SNARE (soluble N-ethylmaleimide-sensitive factor (NSF) attachment protein receptor) proteins drive membrane fusion at different cell compartments as their core domains zipper into a parallel four-helix bundle. After fusion, these bundles are disassembled by the AAA+ (ATPase associated with diverse cellular activities) protein Sec18/NSF and its adaptor Sec17/α-SNAP to make them available for subsequent rounds of membrane fusion. The disassembly requires multiple ATP hydrolysis events in the presence of Mg2+; as few as six ATP hydrolysis events are sufficient. The side-loading and side-release mechanism explains how Sec18/NSF can disassemble SNAREs with constrained topologies.

Next, we asked whether this same side opening of Sec18 occurs in the hydrolyzing condition without SNARE substrate. We prepared purified wild-type Sec18 in the presence of ATP and Mg2+ in a three-stage procedure that yielded a pure sample used for cryo-EM studies. Two bands were visible in native gels, indicating two oligomeric states. Processing and classification led to three classes, two of which appeared to be heptameric and identical (280,935 particles and 73,253 particles, respectively) and a third class that contained indeterminate density in the D1 ring (70,513 particles). Density for the N domains was not well resolved in any of the classes, presumably because of the conformational flexibility of the N domains without substrate or adaptor present. The heptameric class is nearly identical to class 4 observed in the y20S complex under hydrolyzing conditions. Each protomer in the heptamer is similar to the others, with an average r.m.s.d. < 1 Å between them and the angle between the D1 and D2 rings varying only within a small range of 61.9°–67.1°, in contrast to the hexamer, with a range of 60.8°–92.3°. The D1 pore diameter is 30 Å, larger than that of substrate-bound hexamer, with a diameter of ~11 Å. The substrate-free structures (hexamer and heptamer) are nearly identical (r.m.s.d. = 0.48 Å) to the substrate-released structures.

>[7x]GAHMFKIPGFGKAAANHTPPDMTNMDTRTRHLKVSNCPNNSYALANVAAVSPNDFPNNIYIIIDNLFVFTTRHSNDIPPGTIGFNGNQRTWGGWSLNQDVQAKAFDLFKYSGKQSYLGSIDIDISFRARGKAVSTVFDQDELAKQFVRCYESQIFSPTQYLIMEFQGHFFDLKIRNVQAIDLGDIEPTSAVATGIETKGILTKQTQINFFKGRDGLVNLKSSNSLRPRSNAVIRPDFKFEDLGVGGLDKEFTKIFRRAFASRIFPPSVIEKLGISHVKGLLLYGPPGTGKTLIARKIGTMLNAKEPKIVNGPEILSKYVGSSEENIRNLFKDAEAEYRAKGEESSLHIIIFDELDSVFKQRGSRGDGTGVGDNVVNQLLAKMDGVDQLNNILVIGMTNRKDLIDSALLRPGRFEVQVEIHLPDEKGRLQIFDIQTKKMRENNMMSDDVNLAELAALTKNFSGAEIEGLVKSASSFAINKTVNIGKGATKLNTKDIAKLKVTREDFLNALNDVTPAFGISEEDLKTCVEGGMMLYSERVNSILKNGARYVRQVRESDKSRLVSLLIHGPAGSGKTALAAEIALKSGFPFIRLISPNELSGMSESAKIAYIDNTFRDAYKSPLNILVIDSLETLVDWVPIGPRFSNNILQMLKVALKRKPPQDRRLLIMTTTSAYSVLQQMDILSCFDNEIAVPNMTNLDELNNVMIESNFLDDAGRVKVINELSRSCPNFNVGIKKTLTNIETARHDEDPVNELVELMTQSA>MIETPYYLIDKAKLTRNMERIAHVREKSGAKALLALKCFATWSVFDLMRDYMDGTTSSSLFEVRLGRERFGKETHAYSVAYGDNEIDEVVSHADKIIFNSISQLERFADKAAGIARGLRLNPQVSSSSFDLADPARPFSRLGEWDVPKVERVMDRINGFMIHNNCENKDFGLFDRMLGEIEERFGALIARVDWVSLGGGIHFTGDDYPVDAFSARLRAFSDRYGVQIYLEPGEASITKSTTLEVTVLDTLYNGKNLAIVDSSIEAHMLDLLIYRETAKVLPNEGSHSYMICGKSCLAGDVFGEFRFAEELKVG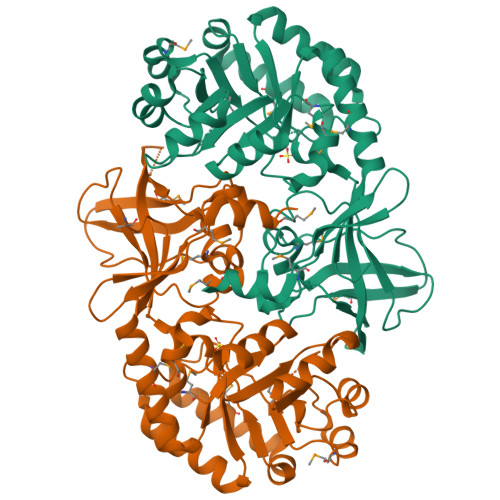DRISFQDAAGYTMVKKNWFNGVKMPAIAIRELDGSVRTVREFTYADYEQSLS[2x]> MDIYGTARAVTTCRMCGAQDWQEVVDFGPVPLADSFLEPAASYDDEPRYPLAVVSCRSCRLMSLTHVVDPEVLYRTYPYTTSDSETIKKHMGHVVAVCVERFGIPEGSFVLEIGSNTGSQLKAFQNAGMRTLGIDPARNIAAVANERGIETLPEFFSVDTAALVKKT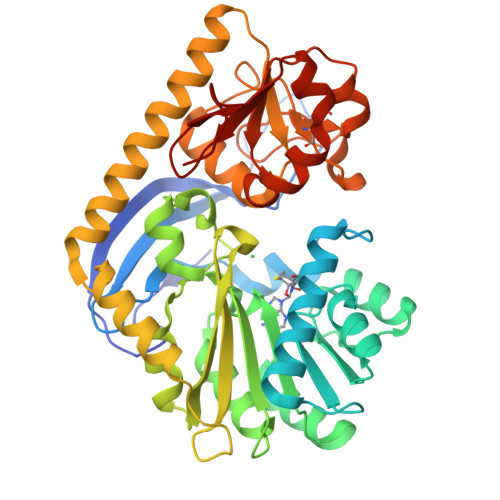HGTPQLVLGRHVFAHIDDVSAVAEGVRDLLGPDSLFAIEVPYLVDMLERNEFDTIYHEHLSYIGVGSLVALFRRHGLRVVDVERLAVHGGSILVFVGLDEGTRATAPVVEELIALEKERGLYEDATYERFARHVAEITAELTSMVRSLRAEGKRIAGYGAPAKGNTLLNVCGLTADDLEFCCDTTEFKQGLVLPGTHIPVRSPEYAKTQAIDYYLLLAWNYGEEILAKEGPFLADGGRFILPNPRPSIVPPGEHHHHHH> SNILEMTKNYYDRSVSPVEYAYFDQSQNMRAINWNKIVDEKDLEVWNRVTQNFWLPENIPVSNDLPSWNELDDDWQQLITRTFTGLTLLDTVQSSIGDVAQIKNSLTEQEQVIYANFAFMVGVHARSYGTIFSTLCTSEQIEEAHEWVVDNEALQARPKALIPFYTADDPLKSKIAAALMPGFLLYGGFYLPFYLSARGKLPNTSDIIRLILRDKVIHNFYSGYKYQLKVAKLSPEKQAEMKQFVFDLLDKMIGLEKTYLHQLYDGFGLADEAIRFSLYNAGKFLQNLGYE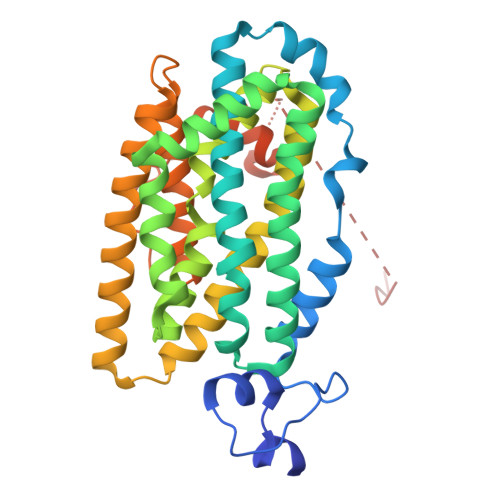SPFTKEETRIAPEVFAQLSARADENHDFFSGSGSSYIIGTSEETLDEDWDF> MENTENSVDSKSIKNL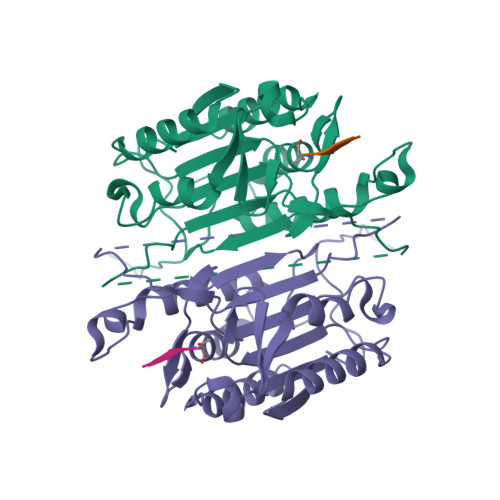EPKIIHGSESMDSGISLDNSYKMDYPEMGLCIIINNKNFHKSTGMTSRSGTDVDAANLRETFRNLKYEVRNKNDLTREEIVELMRDVSKEDHSKRSSFVCVLLSHGEEGIIFGTNGPVDLKKITNFFRGDRCRSLTGKPKLFIIQACRGTELDCGIETDSGVDDDMACHKIPVEADFLFAYSTAPGYYSWRNSKDGSWFIQSLCAMLKQYADKLEFMHILTRVNRKVATEFESFSFDATFHAKKQIPCIVSMLTKELYFYHL4-carbamimidamidobenzoic acid | C8 H9 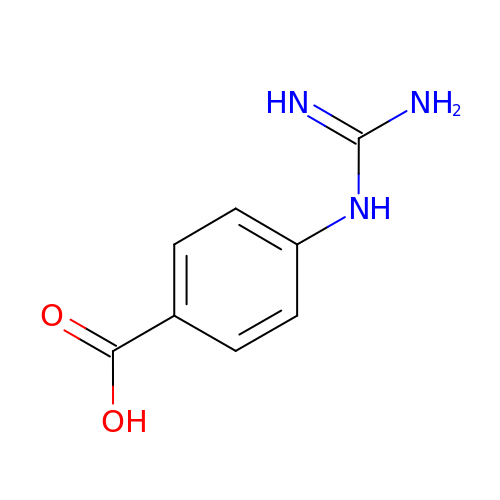N3 O2 | SXTSBZBQQRIYCU-UHFFFAOYSA-N>[2x]SNAMADEIAKAQVARPGGDTIFGKIIRKEIPAKIIFEDDRCLAFHDISPQAPTHFLVIPKKHISQISVAEDDDESLLGHLMIVGKKCAADLGLNKGYRMVVNEGSDGGQSVY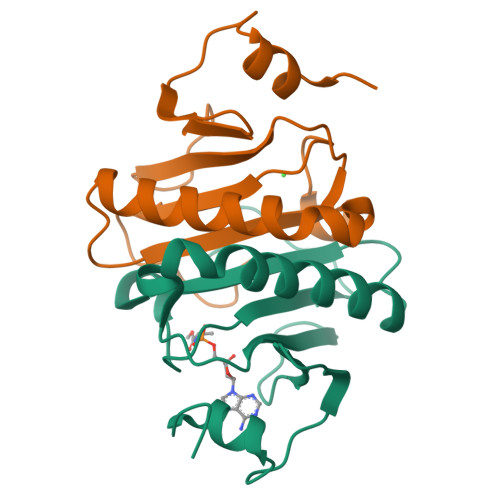HVNLHVLGGRQMHWPPG>KPFTVPILTVEEMTNSRFPIPLEKLFTGPSGAFVVQPQNGRCTTDGVLLGTTQLSPVNICTFRGDVTHIAGTHNYTMNLASQNWNNYDPTEEIPAPLGTPDFVGRIQGMLTQTTRGDGSTRGHKATVSTGDVHFTPKLGSIQFNTDTNNDFETGQNTKFTPVGVVQDGNGAHQNEPQQWVLPSYSGRTGHNVHLAPAVAPTFPGEQLLFFRSTMPGCSGYPNMNLDCLLPQEWVQHFYQEAAPAQSDVALLRFVNPDTGRVLFECKLHKSGYVTVAH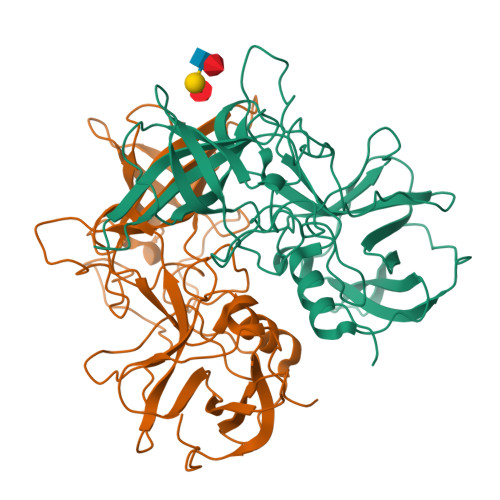TGQHDLVIPPNGYFRFDSWVNQFYTLAPM[2x]>MSFEGKIALVTGASRGIGRAIAELLVERGACVIGTATSEKGAEAISAYLGENGKGLMLNVVDPTSIDTVLATIRAEFGEVDILVNNAGITRDNLLMRMKDDEWQDIIDTNLTSVFRLSKAVMRAMMKKRFGRIITIGSVVGTMGNAGQVNYAAAKAGVIGFSKSLAREVASRGITVNVVAPGFIETDMTRTLTDDQRAGILAQVPANRLGDAKEIASAVAFLASDEASYISGETLHVNGGMYMI[4x]

Ketoacyl-acyl carrier protein reductases (FabG; EC 1.1.1.100) are highly conserved and ubiquitously expressed enzymes of the bacterial type II fatty acid synthesis (FASII) pathway, catalysing the reduction of the acyl carrier protein (ACP) linked β-ketoacyl molecules to β-hydroxyacyl-ACP thioesters necessary for the formation of saturated and unsaturated fatty acids. FabG enzymes are members of the short-chain alcohol dehydrogenase/reductase (SDR) family (also known as the short chain oxidoreductase or SCOR family). The refined structures of the two crystal forms of YpFabG reveal that the protein contains a typical Rossmann fold motif, comprised of a seven strand twisted β-sheet surrounded by eight α-helices. The YpFabG tetramer is formed through two types of interfaces.

YpFabG crystallised in the presence of NaBr (YpFabG NaBr) diffracted to 2.85 Å and contained a homotetramer in the ASU, with electron density visible for 832 of 976 residues, with disordered regions between residues 139–147 and 185–206 in each monomer, and was refined to Rwork/Rfree values of 0.214/0.248. Despite very similar crystallisation conditions, the YpFabG TMAO crystal displays P42212 symmetry with a single YpFabG monomer within the ASU, whereas the YpFabG NaBr crystal displays P1211 symmetry with four YpFabG monomers within the ASU arranged to form a homotetramer. Conversely, this helix-turn-helix motif is completely disordered in our YpFabG NaBr structure. In contrast, a greater portion of the helix-turn-helix motif is disordered in the YpFabG NaBr structure, with little visible electron density in this region. Furthermore, the loop joining β-strand β5 and α-helix α5 within the YpFabG NaBr structure is largely disordered, with superposition of NADP+ bound and unbound E. coli FabG structures indicating that Ser138 located at the start of this loop region must move ~3 Å to accommodate the nicotinamide portion of NADP+. A single phosphate molecule is observed within the same location in our YpFabG NaBr structure, however the presence of this molecule in only one monomer may not be sufficient to induce this active conformation. The only obvious difference between the two tetramers is the presence of the loop joining β-strand β5 and α-helix α5 (residues 139–147), and the helix-turn-helix motif (residues 185–205) in the YpFabG TMAO structure, which are largely disordered in the YpFabG NaBr structure. These regions appear to alter crystal packing, with symmetry generated YpFabG TMAO tetramers packing in parallel, and the helix-turn-helix motifs of each monomer packing against the same motif of the symmetry mate, whilst symmetry mates of the YpFabG NaBr structure appear to form crystal contacts primarily through helices α1, α2, and α3 at the corner of each tetramer. Overall, the structures were similar, with an RMSD of 0.35 Å over 205 amino acids, however they also contained some important structural differences.>[4x]MKYILVTGGVISGVGKGVIASSFGTLLKSCGLDVTSIKIDPY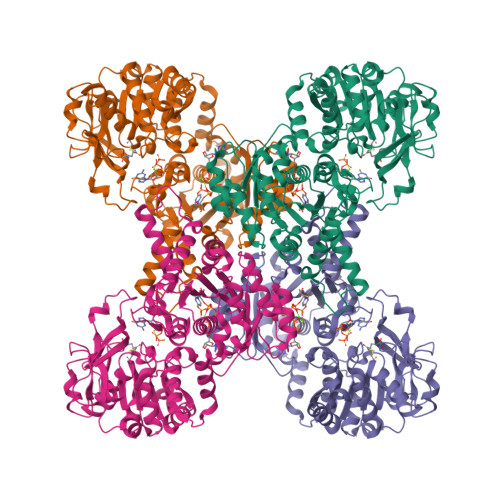INIDAGTFSPYEHGEVYVLDDGAEVDLDLGNYERFLDVTLHRDNNITTGKIYKLVIEKERTGEYLGKTVQVVPHITDAIQEWVERVAQTPVQGSSKPQVCIVELGGTIGDIEGMPFVEAFRQFQFRVKRENFCLAHVSLVPLPKATGEPKTKPTQSSVRELRGCGLSPDLIVCRSEKPIGLEVKEKISNFCHVGPDQVICIHDLNSIYHVPLLMEQNGVIEYLNERLQLNIDMSKRTKCLQQWRDLARRTETVRREVCIAVVGKYTKFTDSYASVVKALQHAALAVNRKLELVFIESCLLEEETLHSEPSKYHKEWQKLCDSHGILVPGGFGSRGMEGKIRACQWARENQKPLLGICLGLQAAVIEFARNKLGLKDANTTEIDPNTANALVIDMPEHHTGQLGGTMRLGKRITVFSDGPSVIRQLYGNPKSVQERHRHRYEVNPKYVHLLEEQGMRFVGTDVDKTRMEIIELSGHPYFVATQYHPEYLSRPLKPSPPFLGLILASVDRLNQYIQRGCRLSPRQLSDASSDEEDSVVGLAGATKSLSSLKIPITPTNGISKSCNGSISTSDSEGACGGVDPTNGHK(2~{R})-2-[(4~{S})-6-(4-chlorophenyl)-8-methoxy-1-methyl-4~{H}-[1,2,4]triazolo[4,3-a][1,4]benzodiazepin-4-yl]-~{N}-ethyl-pent-4-enamide | C25 H26 Cl N5 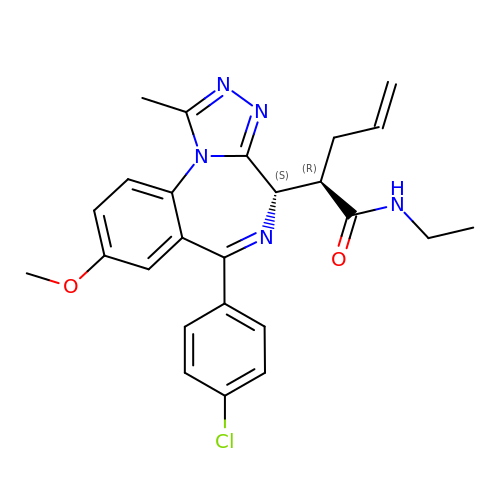O2 | BBDSCBLVVIKKIF-XXBNENTESA-N> MSNISRQAYADMFGPTVGDKVRLADTELWIEVEDDLTTYGEEVKFGGGKVIRDGMGQGQMLAADCVDLVLTNALIVDHWGIVKADIGVKDGRIFAIGKAGNPDIQPNVTIPIGAATEVIAAEGKIVTAGGIDTHIHWICPQQAEEALVSGVTTMVGGGTGPAAGTHATTCTPGPWY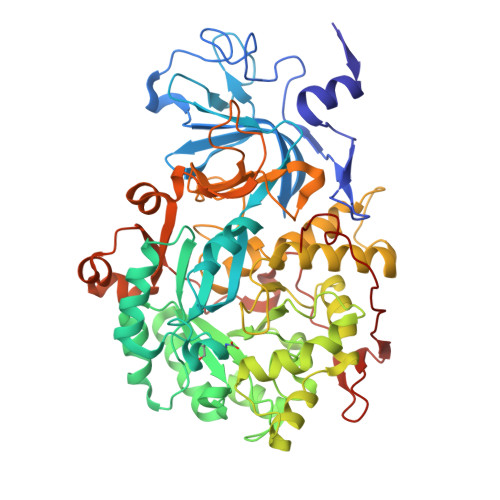ISRMLQAADSLPVNIGLLGKGNVSQPDALREQVAAGVIGLKINEDWGATPAAIDCALTVADEMDIQVALHSDTLNESGFVEDTLAAIGGRTIHTFHTEGAGGGHAPDIITACAHPNILPSSTNPTLPYTLNTIDEHLDMLMVCHHLDPDIAEDVAFAESRIRRETIAAEDVLHDLGAFSLTSSDSQAMGRVGEVILRTWQVAHRMKVQRGALAEETGDNDNFRVKRYIAKYTINPALTHGIAHEVGSIEVGKLADLVVWSPAFFGVKPATVIKGGMIAIAPMGDINASIPTPQPVHYRPMFGALGSARHHCRLTFLSQAAAANGVAERLNLRSAIAVVKGCRTVQKADMVHNSLQPNITVDAQTYEVRVDGELITSEPADVLPMAQRYFLF> MDAEPKRKFGVVVVGVGRAGSVRLRDLKDPRSAAFLNLIGFVSRRELGSLDEVRQISLEDALRSQEIDVAYICSESSSHEDYIRQFLQAGKHVLVEYPMTLSFAAAQELWELAAQKGRVLHEEHVELLMEEFEFLRREVLGKELLKGSLRFTASPLEEERFGFPAFSGISRLTWLVSLFGELSLISATLEERKEDQYMKMTVQLETQNKGLLSWIEEKGPGLKRNRYVNFQFTSGSLEEVPSVGVNKNIFLKDQDIFVQKLLDQVSAEDLAAEKKRIMHCLGLASDIQK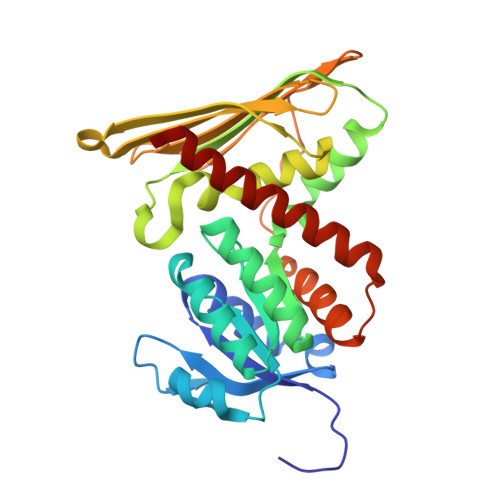LCHQKK> MAQTPAFDKPKVELHVHLDGAIKPETILYYGKRRGIALPADTPEELLNIIGMDKPLTLPDFLAKFDYYMPAIAGCRDAIKRIAYEFVEMKAKDGVVYVEVRYSPHLLANSKVEPIPWNQAEGDLTPDEVVSLVNQGLQEGERDFGVKVRSILCCMRHQPSWSSEVVELCKKYREQTVVAIDLAGDETIEGSSLFPGHVQAYAEAVKSGVHRTVHAGEVGSANVVKEAV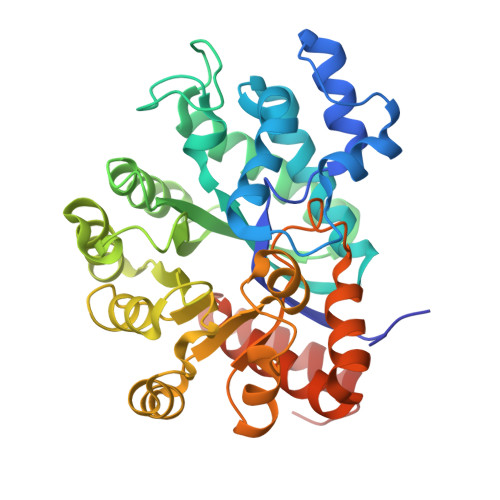DTLKTERLGHGYHTLEDTTLYNRLRQENMHFEICPWSSYLTGAWKPDTEHAVIRFKNDQVNYSLNTDDPLIFKSTLDTDYQMTKKDMGFTEEEFKRLNINAAKSSFLPEDEKKELLDLLYKAYRMPSPASAEQCL> SNKKMINGGTVN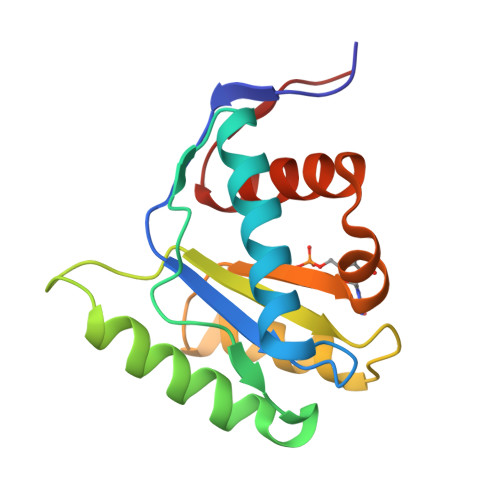NWICINFSRQVQDNLARTFCQELAQMCYVSGMAFNPEPVLPPVSARPEQVEKVLKTRYHDATSKLSQGKEIDLLIVILPDNNGSLYGDLKRICETELGIVSQCCLTKHVFKMSKQYMANVALKINVKVGGRNTVL6-(4-{[3-(2,6-dichlorophenyl)-5-(1-methylethyl)isoxazol-4-yl]methoxy}phenyl)quinoline-2-carboxylic 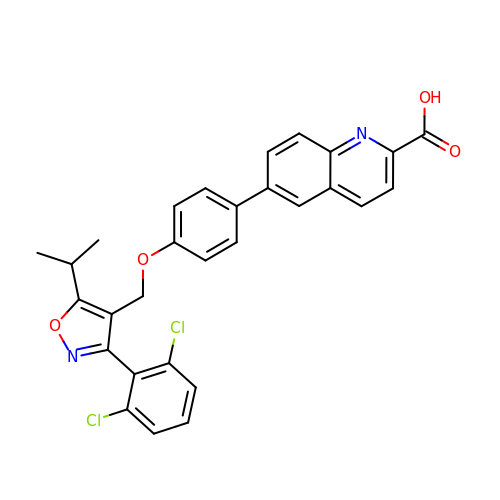acid | C29 H22 Cl2 N2 O4 | SZUHDKKQQZPOGX-UHFFFAOYSA-N> ACDYTCGSNCYSSSDVSTAQAAGYKLHEDGETVGSNSYPHKYNNYEGFDFSVSSPYYEWPILSSGDVYSGGSPGADRTVFN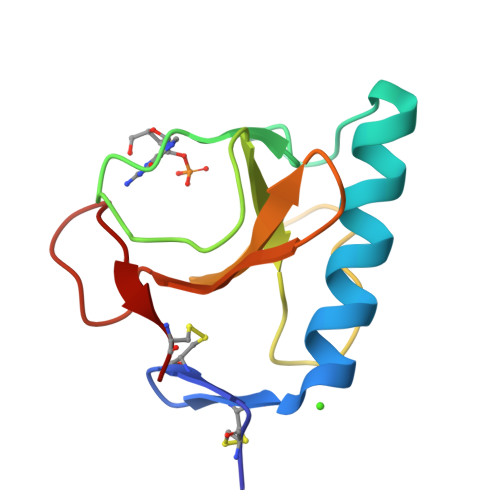ENNQLAGVITHTGASGNNFVECT>AWKVSVDQDTCIGDAICASLCPDVFEMNDEGK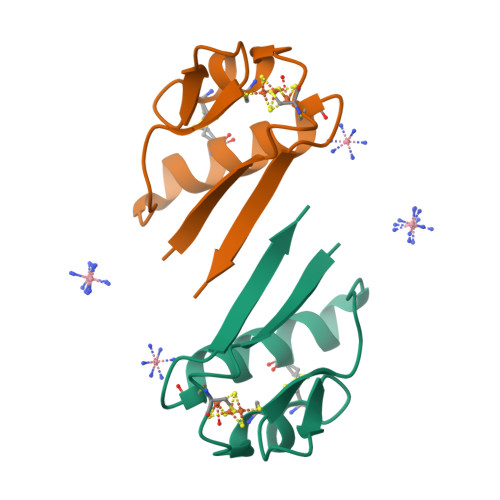AQPKVEVIEDEELYNCAKEAMEACPVSAITIEEA[2x]> MSSFYTVVGVFIVVSAMSVLFWIMAPKNNQAVWRSTVILTLAMM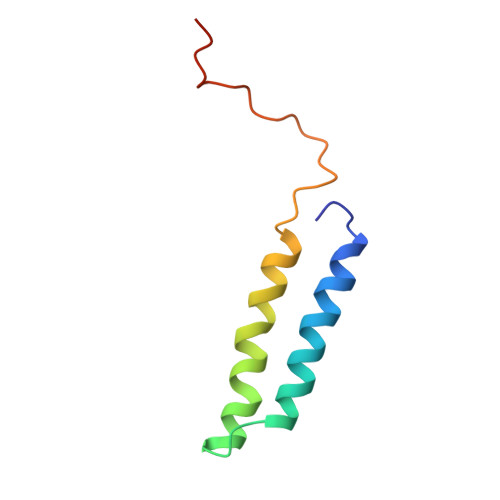FLMWAITFLCQLHPLVAPRRSDLRPEFAE> XGELKAIAQELKAIAYELKAI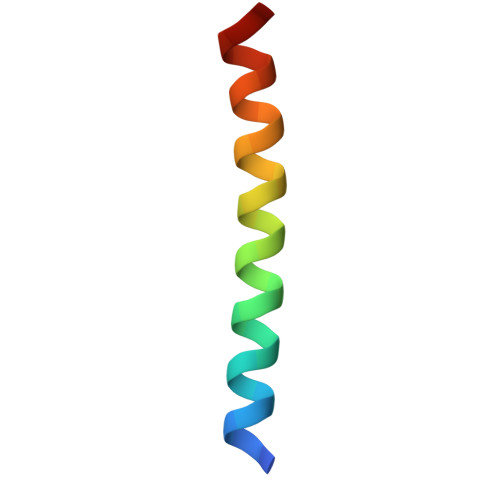AKEDKAIAQGX Serial femtosecond crystallography (SFX) using ultrashort pulses from X-ray free-electron lasers (XFELs) can overcome typical radiation damage to protein crystals via the “diffraction-before-destruction” approach. Here we introduce hydroxyethyl cellulose (cellulose matrix) for serial sample loading. We demonstrate the cellulose matrix as a protein carrier for SFX using small and large sized crystals (1 × 1 × 1 to 20 × 20 × 30 μm). In addition, we demonstrate the successful de novo phasing in SFX by applying praseodymium (Pr)-SAD, single-isomorphous replacement (SIR) and SIR with anomalous scattering (SIRAS) phasing to determine the structure of proteinase K. Furthermore, to reduce background scattering, a novel grease matrix, Super Lube nuclear grade grease (nuclear grease), was introduced in this study.

Using lysozyme (1 × 1 × 1 μm) and thaumatin (2 × 2 × 4 μm) crystals dispersed in a cellulose matrix, we were able to collect 100,000–150,000 images in approximately 60–80 min at a wavelength of 1.24 Å. At a flow rate of 0.43 and 0.47 μl min−1, a total sample volume of about 30–40 μl was used with a crystal number density of 5.8 × 108 crystals ml−1 for lysozyme, and 4.3 × 108 crystals ml−1 for thaumatin. We indexed and integrated 30,000–40,000 images for both the lysozyme (space group P43212) and thaumatin (space group P41212) crystals. The lysozyme and thaumatin crystals yielded data sets at 1.8-Å and 1.55-Å resolution with a completeness of 100% and a CC1/2 of 0.992 and 0.988, respectively. In this study, 16% (w/v) and 22% (w/v) cellulose matrices were used for the small sized lysozyme (1 × 1 × 1 μm) and thaumatin (2 × 2 × 4 μm) crystals, respectively. The cellulose matrix with randomly oriented crystals was extruded through an injector nozzle with an inner diameter (i.d.) of 50 μm.

> ATFEIVNRCSYTVWAAASKGDAALDAGGRQLNSGESWTINVEPGTNGGKIWARTDCYFDDSGSGICKTGDCGGLLRCKRFGRPPTTLAEFSLNQYGKDYIDISNIKGFNVPMDFSPTTRGCRGVRCAADIVGQCPAKLKAPGGGCNDACTVFQTSEYCCTTGKCGPTEYSRFFKRLCPDAFSYVLDKPTTVTCPGSSNYRVTFCPTA PHENYL-URIDINE-5'-DIPHOSPHATE | C15 H18 N2 O12 P2 | 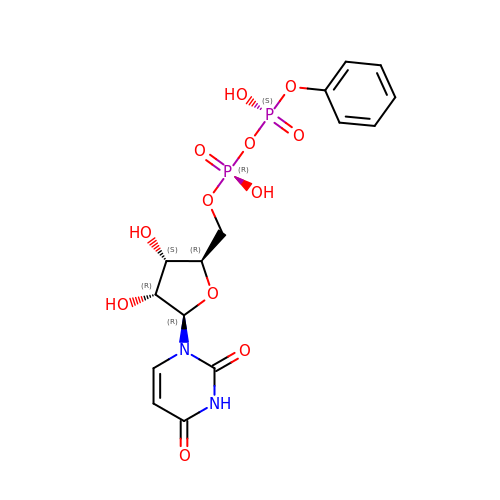ZHUWBKDWWGKIEN-FMKGYKFTSA-N Type III secretion systems (T3SS) are bacterial macromolecular machines that facilitate transport of protein substrates across the bacterial cell envelope. Most building blocks of the virulence associated T3SS or injectisome have a homologue in flagella and one of the most highly conserved parts of the system is a set of transmembrane proteins known collectively as the export apparatus (EA). The FlhA/SctV cytoplasmic domain is known to form a nonameric ring underneath FliPQR-FlhB/SctRSTU, but the full-length FlhA/SctV complex remains poorly characterised. Open and closed states have been described, with the open state being competent for chaperone-substrate complex binding, while the closed state has been proposed to be responsible for binding early substrates.

Out of the identified proteins we chose FlhA from the lateral flagella of Vibrio parahaemolyticus (Vp-FlhA) and SctV from Yersinia enterocolitica (Ye-SctV) for further studies, as both could be produced in large quantities at high purity using the gentle detergent LMNG. Particle classification revealed that Ye-SctV had formed a dimer of nonamers and we imposed D9 symmetry for 3D refinement, resulting in a 3.7 Å reconstruction of the cytoplasmic domain double nonamer. The Ye-SctV cytoplasmic domain 18-mer is made up of two nonamers dimerising via the cytoplasm facing side of the cytoplasmic domain. This assembly is not consistent with the known localisation of SctV in the injectisome and is therefore considered to be an artefact of the removing the complex from the constraint of the membrane. No high-resolution features of the transmembrane domain could be discerned. A striking feature of both structures is the N-terminal density of the cytoplasmic domain, formed by FlhAL/SctVL, which reaches out to bind to the adjacent protomer, demonstrating this well studied interaction for the first time in the context of the full-length protein in both flagellar and injectisome T3SS. In both of our structures a hydrophobic residue, Trp350 in Vp-FlhA and Phe367 in Ye-SctV, sticks into a hydrophobic groove on the neighbouring subunit. Comparison of our structures with FlhA from S. Typhimurium, St-FlhA, in the open state and Sf-SctV, which is in the closed state shows that both of our complexes are in the open state, with Ye-SctV being the first example of an SctV homologue in the open state. The demonstration of the open state opens up the possibility that SctV binds to substrate-chaperone complexes in an analogous manner to that described for FlhA, in which chaperones bind between Sub-Domain(SD)4 and SD2 and are sterically unable to access the binding site in the closed state. While molecular dynamics simulations suggested that E. coli SctV does not easily switch between open and closed state, our SctV and the C. pneumoniae SctV structure show that SctV can exist in the open state.

>[18x]MNPHDLEWLNRIGERKDIMLAVLLLAVVFMMVLPLPPIVLDILIAVNMTISVVLLMIAIYINSPLQFSAFPAVLLVTTLFRLALSVSTTRMILLQADAGQIVYTFGNFVVGGNLIVGIVIFLIITIVQFLVITKGSERVAEVSARFSLDAMPGKQMSIDGDMRAGVIDVNEARERRATIEKESQMFGSMDGAMKFVKGDAIAGLIIIFVNILGGVTIGVTQKGLAAAEALQLYSILTVGDGMVSQVPALLIAITAGIIVTRVSSEDSSDLGSDIGKQVVAQPKAMLIGGVLLLLFGLIPGFPTVTFLILALLVGCGGYMLSRKQSRNDEANQDLQSILTSGSGAPAARTKAKTSGANKGRLGEQEAFAMTVPLLIDVDSSQQEALEAIALNDELVRVRRALYLDLGVPFPGIHLRFNEGMGEGEYLISLQEVPVARGELKAGYLLVRESVSQLELLGIPYEKGEHLLPDQETFWVSVEYEERLEKSQLEFFSHSQVLTWHLSHVLREYAEDFIGIQETRYLLEQMEGGYGELIKEVQRIVPLQRMTEILQRLVGEDISIRNMRSILEAMVEWGQKEKDVVQLTEYIRSSLKRYICYKYANGNNILPAYLFDQEVEEKIRSGVRQTSAGSYLALDPAVTESLLEQVRKTIGDLSQIQSKPVLIVSMDIRRYVRKLIESEYYGLPVLSYQELTQQINIQPLGRVCLENLYFQ> MDSTNLNKRPLLQYSLSSLGSQITKWSSSRPTSPVRKARSTENDFLSKQDTSSILPSINDDGGEQWYEKFKPNCLEQVAIHKRKLKDVQEALDAMFLPNAKHRILLLSGPSGCSKSTVIKELSKILVPKYRQNSNGTSFRSTPNEHKVTEFRGDCIVNDLPQMESFSEFLKGARYLVMSNLSLILIEDLPNVFHIDTRRRFQQLILQWLYSSEPLLPPLVICITECEIPENDNNYRKFGIDYTFSAETIMNKEILMHPRLKRIKFNPINSTLLKKHLKFICVQNMKMLKEKNKWNKRQEVIDYIAQETGDIRSAITTLQFWATSSGSLPISTRESTISYFHAIGKVIHGSHSTNNDNEMINNLFENSNNLLSKEDFKLGILENYNTFNKGEFSISDASSIVDCLSECDNMNGLPESNEYGLREVRKTFRNISKQGHNHGTVYFPREWKVRKLQNSFKVQAEDWL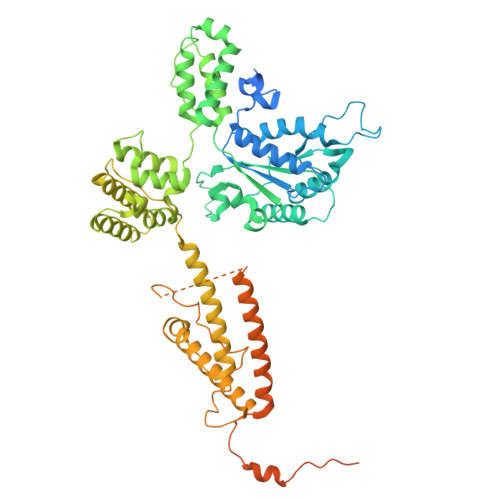NVSLYKYNAVHSFRNITLEFGYYAPLIRKCQSYKKKYILYYLKNLPSGSSGPKQTMDKFSDIMKVENGIDVVDRIGGPIEALSVEDGLAPLMDNDSNNCDHLEDQKKERDRRLRMLIDQYERNVMMANDDLEDEETSFNDDPIVDSDSDNSNNIGNETFGRSDEDESLCEILSQRQPRKAPVISESLSDSDLEILGLNLEVLFQGPGGDYKDDDDKDYKDDDDKDYKDDDDK>[2x]MAVTDLSL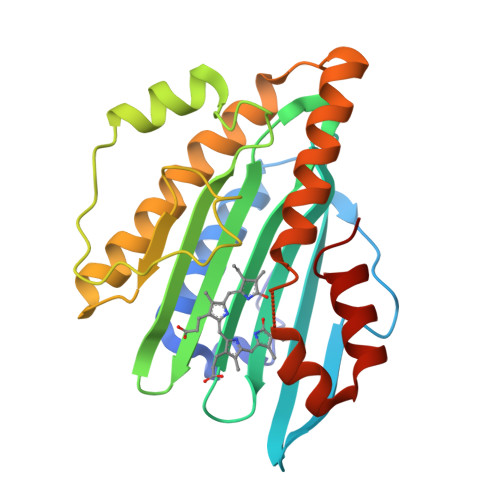TNSSLMPTLNPMIQQLALAIAASWQSLPLKPYQLPEDLGYVEGRLEGEKLVIENRCYQTPQFRKMHLELAKVGKGLDILHCVMFPEPLYGLPLFGCDIVAGPGGVSAAIADLSPTQSDRQLPAAYQKSLAELGQPEFEQQRELPPWGEIFSEYCLFIRPSNVTEEERFVQRVVDFLQIHCHQSIVAEPLSEAQTLEHRQGQIHYCQQQQKNDKTRRDLEKAFGEAWAERYMSQVLFDVIQ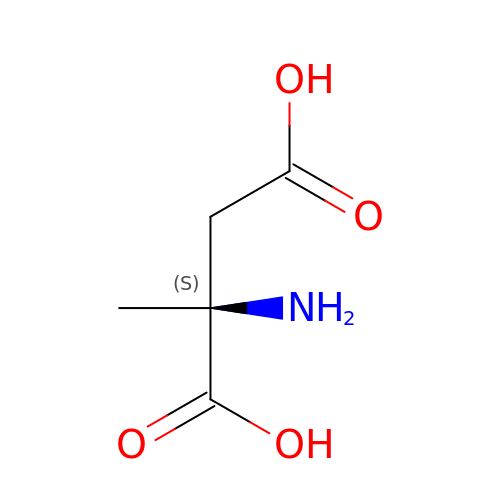2-methyl-L-aspartic acid | C5 H9 N O4 | CWAYDJFPMMUKOI-YFKPBYRVSA-N> NEPAIEAFLQDGGTLAMLNDVSTDTLEQLYTLGFNQYHAGKHDEAHKIFQALCVLDHYEARFFLGLGACRQALGQFRLAIDSYSYGAMMDLQEPRFPFHAAECLLQLGELEGAE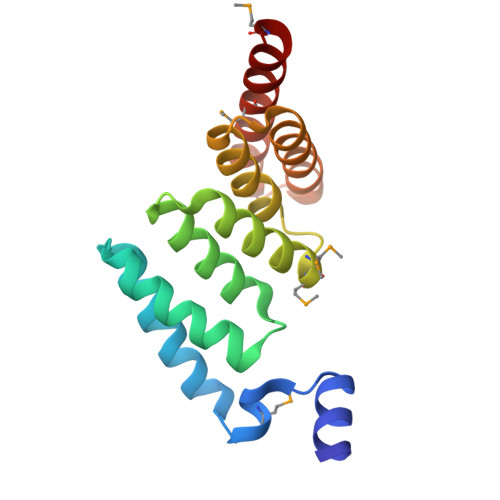SGFHSAQLLAAAKPELAELAARAGIMLEVVKTKKDME>MISLADLQRRIETGELSPNAAIAQSHAAIEAREKEVHAFVRHDKSARAQASGPLRGIAVGIKDIIDTANMPTEMGSEIYRGWQPRSDAPVVMMLKRAGATIIGKTTTTAFASRDPTATLNPHNTGHSPGGSSSGSAAAVGAGMIPLALGTQTGGCVIRPAAYCGTAAIKPSFRMLPTVGVKCYSWALDTVGLFGARAEDLARGLLAMTGRSEFSGIVPAKAPRIGVVRQEFAGAVEPAAEQGLQAAIKAAERAGASVQAIDLPEAVHEAWRIHPIIQDFEAHRALAWEFSEHHDEIAPMLRASLDATVGLTPKEYDEARRIGRRGRRELGEVFEGVDVLLTYSAPGTAPAKALASTGDPRYNRLWTLMGNPCVNVPVLKVGGLPIGVQVIARF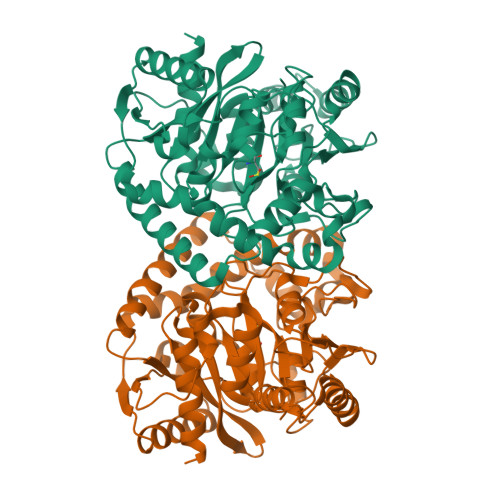GNDAHALATAWFLEDALAKSG[2x]> GA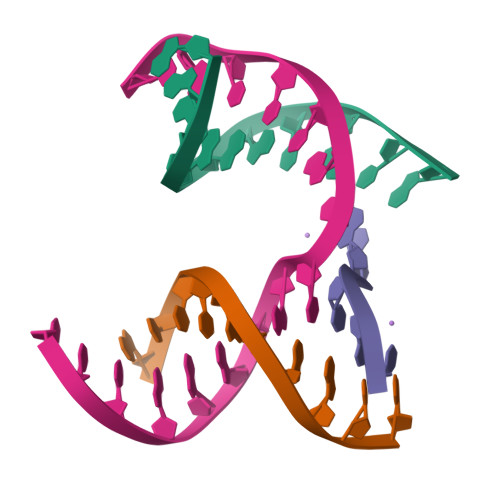GCAGACGTG;> ACAGCACTCA;> CATGT;> TCTGAGTGCCGTCTGC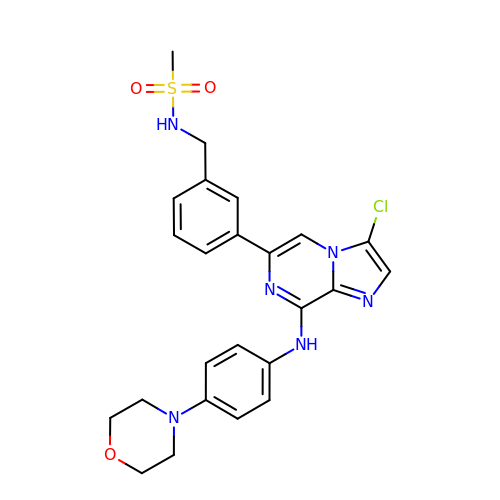N-(3-{3-chloro-8-[(4-morpholin-4-ylphenyl)amino]imidazo[1,2-a]pyrazin-6-yl}benzyl)methanesulfonamide | C24 H25 Cl N6 O3 S | BHSRVQWRAVCUOG-UHFFFAOYSA-N Heat shock factor 1 (HSF1) and 2 (HSF2) play distinct but overlapping regulatory roles in maintaining cellular proteostasis or mediating cell differentiation and development. Upon activation, both HSFs trimerize and bind to heat shock elements (HSEs) present in the promoter region of target genes. HSFs recognize and bind HSEs through the DBD, which is the most conserved and only structurally characterized domain. Here, we present co-crystal structures of human HSF1 and HSF2 trimers bound to DNA, which reveal a triangular arrangement of the three DNA-binding domains (DBDs) with protein-protein interactions largely mediated by the wing domain.

Crystallization of the HSF1 trimer in complex with the same three-site HSE was unsuccessful until longer sticky-ended DNA duplexes were attempted. Two structures containing 23- and 24-bp oligonucleotides were determined and refined at 2.4 and 2.36 Å. Different from the HSF2 structure, two HSF1 trimers bound to two intact HSEs reside in the asymmetric unit in both structures, where the DNA duplexes were stacked in a head-to-head manner. As a consequence, the two HSF1 trimers are differently oriented with a large rotation angle between them, but little conformational discrepancies exist among all the HSF1-HSE copies present in both structures. Like HSF2, Arg117 (corresponding to Arg109 in HSF2) in the middle DBD (DBD II) also inserts into the major groove and forms a direct hydrogen bond with the nucleobase 5′ to TTC. For example, in the structure comprising 23-bp DNA, the C terminus of DBD II in the first trimer is rigidified by a close contact between Lys118 and the phosphate backbone of DNA but not in the other two DBDs. Particularly, the entire loop in an HSF1 trimer bound to the 23 bp DNA was visible and thus used for further analysis. This domain extends toward DBD III without contacting the DNA double helix or DBD II. By contrast, in both HSF1 trimer-binding structures, dramatic bending occurs at both the 5′-proximal HSE triplet and the downstream dinucleotide, although relatively smaller bending occurs at the 3′-proximal nGAAn repeat bound by DBD III.

>[6x]GHHHHHHVPAFLTKLWTLVSDPDTDALICWSPSGNSFHVFDQGQFAKEVLPKYFKHNNMASFVRQLNMYGFRKVVHIEQGGLVKPERDDTEFQHPCFLRGQEQLLENIKRKVT> GAMANLRTYRA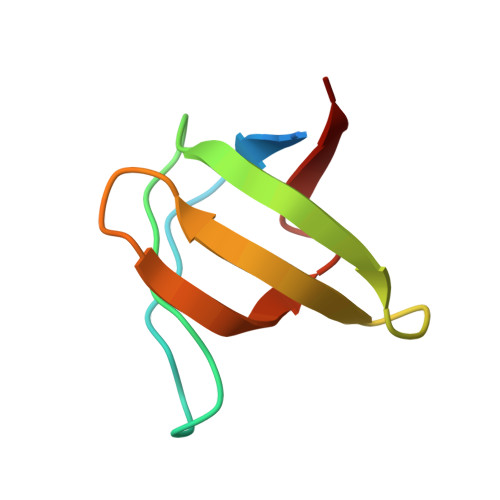MYDYSAQDEDEVSFRDGDYIVNVQPIDDGWMYGTVQRTGRTGMLPANYIEFVN S-{2-[(2-chloro-4-sulfamoylphenyl)amino]-2-oxoethyl} 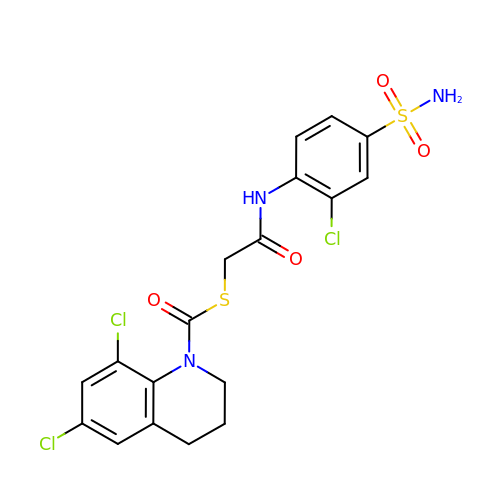6,8-dichloro-3,4-dihydroquinoline-1(2H)-carbothioate | C18 H16 Cl3 N3 O4 S2 | SZLMFNKKFJUHKQ-UHFFFAOYSA-N>MGSSHHHHHHSSGLVPRGSHMERPQLDSMSQDLSEALKEATKEVHIRAENSEFMRNFQKGQVSREGFKLVMASLYHIYTALEEEIERNKQNPVYAPLYFPEELHRRAALEQDMAFWYGPHWQEAIPYTPATQHYVKRLHEVGGTHPELLVAHAYTRYLGDLSGGQVLKKIAQKAMALPSSGEGLAFFTFPSIDNPTKFKQLYRARMNTLEMTPEVKHRVTEEAKTAFLLNIELFEELQALLPEEHKDQSASQTMQTTAPPVKESSFVEKMKKTGRNIIVFYGSQTGTAEEFANRLSKDAHRYGMRGMSADPEEYDLADLSSLPEIDKSLVVFCMATYGEGDPTDNAQDFYDWLQETDVDLTGVKFAVFGLGNKTYEHFNAMGKYVDQRLEQLGAQRIFELGLGDDDGNLEEDFITWREQFWPAVCEFFGVEASSIRQYELVVHEDMDVAKVYTGEMGRLKSYENQKPPFDAKNPFLAAVTANRKLNQGTERHLMHLELDISDSKIRYESGDHVAVYPANDSALVNQIGEILGADLDVIMSLNNLDEESNKKHPFPCPTTYRTALTYYLDITNPPRTNVLYELAQYASEPSEQEHLHKMASSSGEGKELYLSWVVEARRHILAILQDYPSLRPPIDHLCELLPRLQARYYSIASSSKVHPNSVHICAVAVEYEAKSGRVNKGVATSWLRAKEPAGENGGRALVPMFVRKSQFRLPFKSTTPVIMVGPGTGIAPFMGFIQERAWLREQGKEVGETLLYYGCRRSDEDYLYREELARFHKDGALTQLNVAFSREQAHKVYVQHLLKRDREHLWKLIHEGGAHIYVCGDARNMAKDVQNTFYDIVAEFGPMEHTQAVDYVKKLM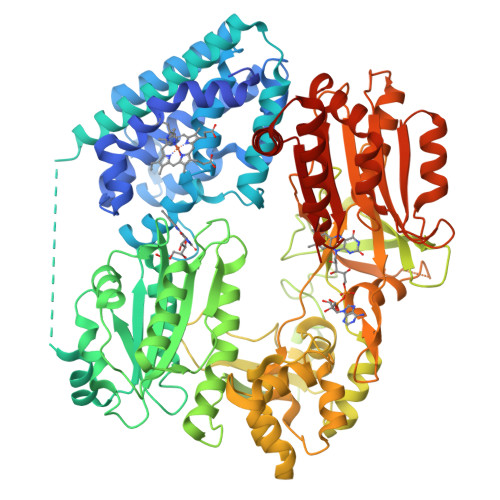TKGRYSLDVWS[2x]>ADTIVAVELDTYPNTDIGDPSYPHIGIDIKSVRSKKTAKWNMQNGKVGTAHIIYNSVGKRLSAVVSYPNGDSATVSYDVDLDNVLPEWVRVGLSASTGLYKETNTILSWSFTSKLKSNSTHETNALHFVFNQFSKDQKDLILQGDATTGTDGNLELTRVSSNGSPQGNSVGRALFYAPVHIWESSAVVASFDATFTFLIKSSDSHPADGIAFFISNIDSSIPS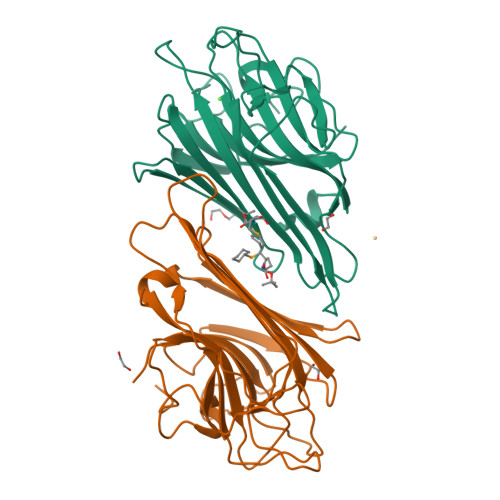GSTGRLLGLFPDAN[2x]> XVALDPIDISIVLNKIKSQLEESKEWIRRSN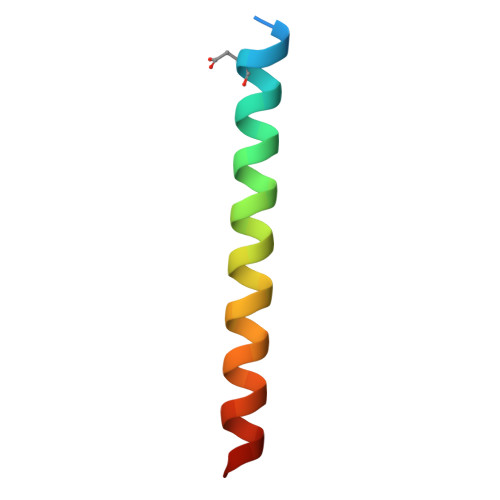KILDSIX> GDFVKPGSLSVKVTDWGNTEYDVTLNLGGTYDWVVKVKLKDGSSVSSFWSANKAEEGGYVVFTP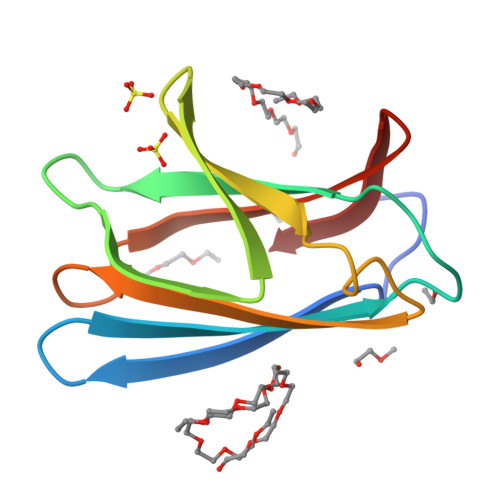VSWNRGPTATFGFIATGSESVEAIYLYVDGQLWDAW>[2x]DYYFPPQKTCLICGDEASGAHYGALTCGSCKVFFKRAAEGKQKYLCASRNDC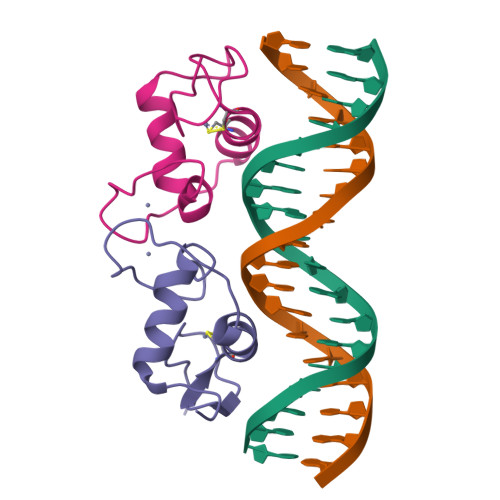TIDKFRRKNCPSCRLRKCYEAGMTLGARKLKKLGNLKLQEEGENSSAGSPTED>[2x]VVGGTRAAQGEFPFMVRLSMGCGGALYAQDIVLTAAHCVSGSGNNTSITATGGVVDLQSSSAVKVRSTKVLQAPGFTKETYGKDWALIKLAQPINQPTLKIAT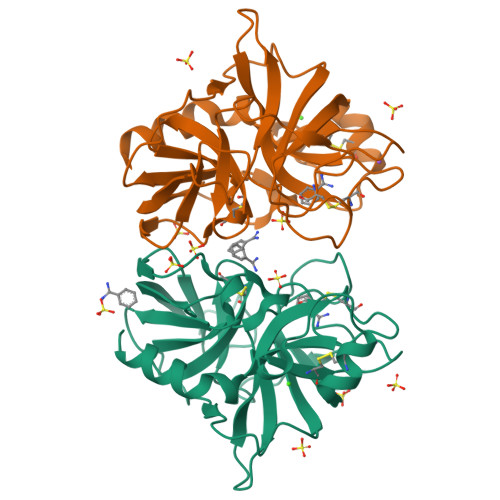TTAYNQGTFTVAGWGANREGGSQQRYLLKANVPFVSDAACRSSSSFILVANEMICAGYDTKQEDTCQGDSGGPMFRKDNADEWVQVGIVSWGEGCARKGKYGVYTEVSTFASAIASAARTL>ASMTTPCITILSGHFPKETIYARKTKELVEEYCSIHGYNFYYEESEPLETEEHALHFRRSWIIQQAAEKFPSTEWFLWLDSDVYVNPKNKNKPITSFIDLSDPNILYHTFHEAPWGSYPINTGVKFVHKDALEIEKIV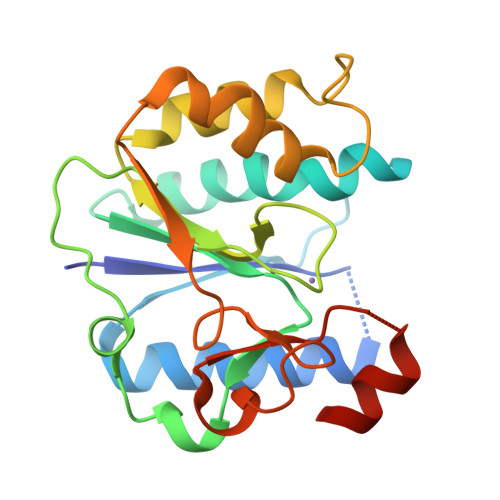WSLRNEAPWNTFPYEQKTVYEYVFPRIPGRYIVHDPYTLNCIVKAYPEHVKDALFVHMCGTSRAERDEHMEMVAT[2x]1,3-dimethyl-8-{[2-(morpholin-4-yl)ethyl]amino}-3,7-dihydro-1H-purine-2,6-dione | C13 H20 N6 O3 | 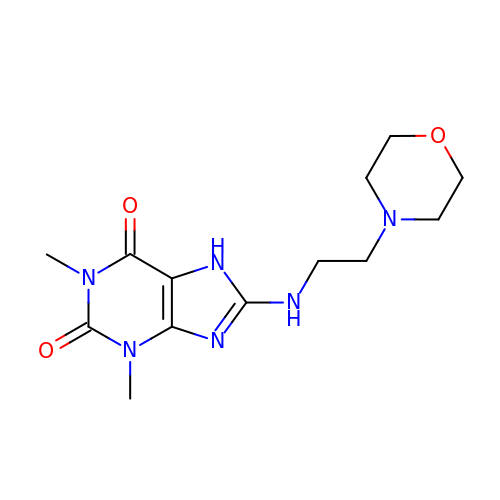BAASUQZVWLHLKR-UHFFFAOYSA-N> MSATK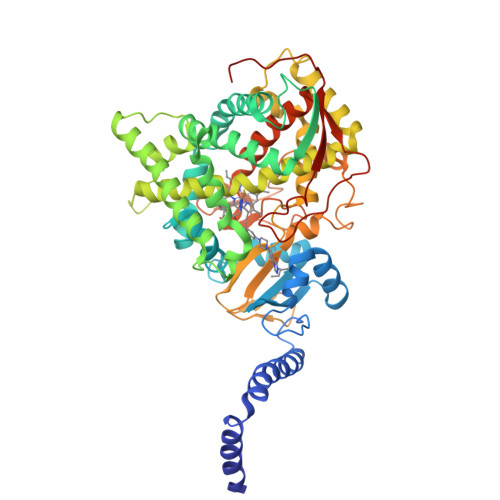SIVGEALEYVNIGLSHFLALPLAQRISLIIIIPFIYNIVWQLLYSLRKDRPPLVFYWIPWVGSAVVYGMKPYEFFEECQKKYGDIFSFVLLGRVMTVYLGPKGHEFVFNAKLADVSAEAAYAHLTTPVFGKGVIYDCPNSRLMEQKKFVKGALTKEAFKSYVPLIAEEVYKYFRDSKNFRLNERTTGTIDVMVTQPEMTIFTASRSLLGKEMRAKLDTDFAYLYSDLDKGFTPINFVFPNLPLEHYRKRDHAQKAISGTYMSLIKERRKNNDIQDRDLIDSLMKNSTYKDGVKMTDQEIANLLIGVLMGGQHTSAAISAWILLHLAERPDVQQELYEEQMRVLDGGKKELTYDLLQEMPLLNQTIKETLRMHHPLHSLFRKVMKDMHVPNTSYVIPAGYHVLVSPGYTHLRDEYFPNAHQFNIHRWNNDSASSYSVGEEVDYGFGAISKGVSSPYLPFGGGRHRCIGEHFAYCQLGVLMSIFIRTLKWHYPEGKTVPPPDFTSMVTLPTGPAKIIWEKRNPEQKIGGRHHHHHH> ASAMFRKLAAESFGTFWLVFGGSGSAVLAAGFPELGIGFAGVALAFGLTVLTMAFAVGHISGGHFNPAVTIGLWA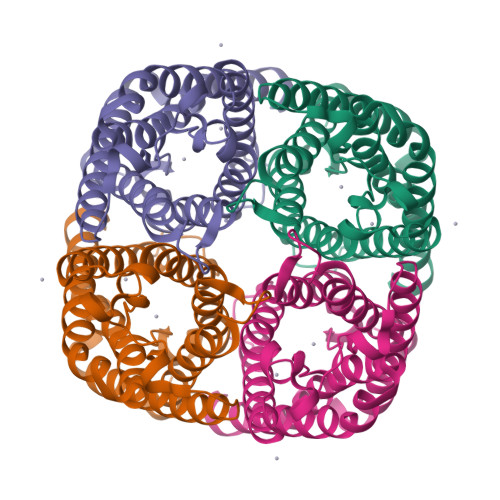GGRFPAKEVVGYVIAQVVGGIVAAALLYLIASGKTGFDAAASGFASNGYGEHSPGGYSMLSALVVELVLSAGFLLVIHGATDKFAPAGFAPIAIGLALTLIHLISIPVTNCSVNPARSTAVAIFQGGWALEQLWFFWVVPIVGGIIGGLIYRTLLEKRD>[2x]GMAINIIEYNRSYKEELIEFILSIQKNEFNIKIDRDDQPDLENIEHNYLNSGGQFWLAINNHQNIVGTIGLIRL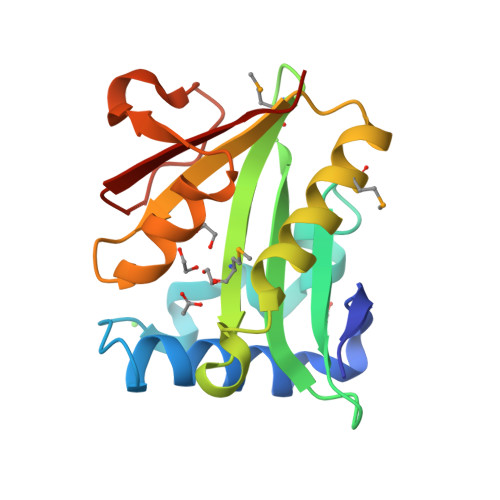DNNMSALKKMFVDKGYRNLKIGKKLLDKVIMTCKEQNIDGIYLGTIDKFISAQYFYSNNGFREIKRGDLPSSFPKLDVDNRFYYRNLKD tert-butyl {(2S)-1-[formyl(hydroxy)amino]-3-phenylpropan-2-yl}carbamate 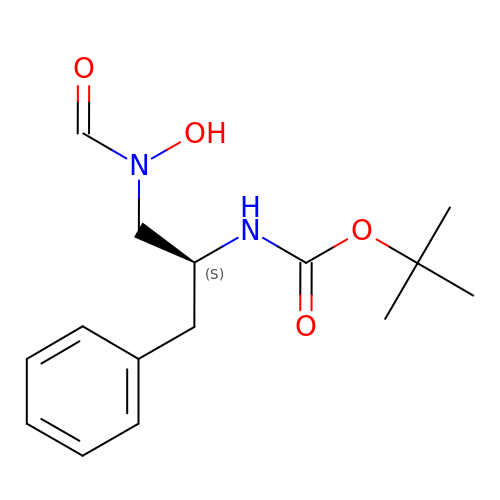| C15 H22 N2 O4 | WLOCWKYZMRXKHU-ZDUSSCGKSA-N> UCCCAGUCCACCG;> CGGUGAGAAGGGXGGCAGAGAAACACACGA;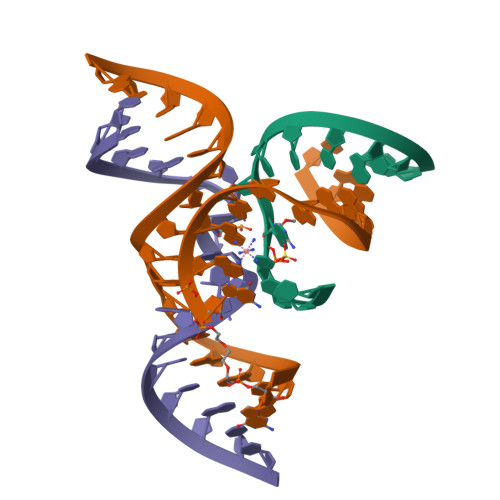> UCGUGGUACAUUACCUGCC> MGSSHHHHHHENLYFQGMKLTTIAKATLALGILTTGVFTAESQTGHAKVELDETQRKYYINMLHQYYSEESFEPTNISVKSEDYYGSNVLNFKQRNKAFKVFLLGDDKNKYKEKTHGLDVFAVPELIDIKGGIYSVGGITKKNVRSVFGFVSNPSLQVKKVDAKNGFSINELFFIQKEEVSLKELDFKIRKLLIEKYRLYKGT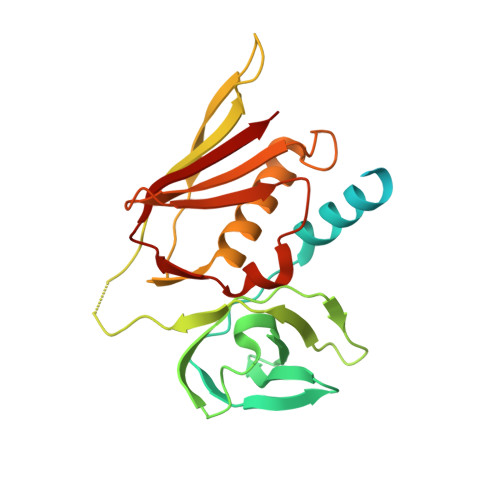SDKGRIVINMKDEKKHEIDLSEKLSFERMFDVMDSKQIKNIEVNLN> MVSLFKRGKA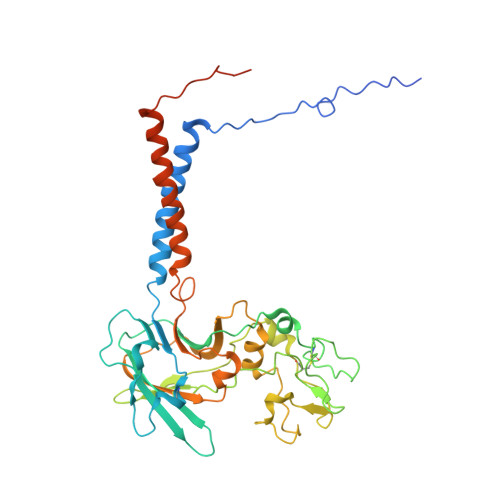PPLTKEGPTSKKPPNTAFRQQRLKAWQPILSPQSVLPLLIFVACIFTPIGIGLIVSATKVQDLTIDYSHCDTKASTTAFEDIPKKYIKYHFKSKVENKPQWRLTENENGEQSCELQFEIPNDIKKSIFIYYKITNFYQNHRRYVQSFDTKQILGEPIKKDDLDTSCSPIRSREDKIIYPCGLIANSMFNDTFSQVLSGIDDTEDYNLTNKHISWSIDRHRFKTTKYNASDIVPPPNWMKKYPDGYTDENLPDIHTWEEFQVWMRTAAFPKFYKLTLKNESASLPKGKYQMNIELNYPISLFGGTKSFVLTTNGAIGGRNMSLGVLYLIVAGLCALFGIIFLVKLIFQPRAMGDHTYLNFDDEENEDYEDVHAENTTLREIL> CGCATATTTGCG;> CGCAAAT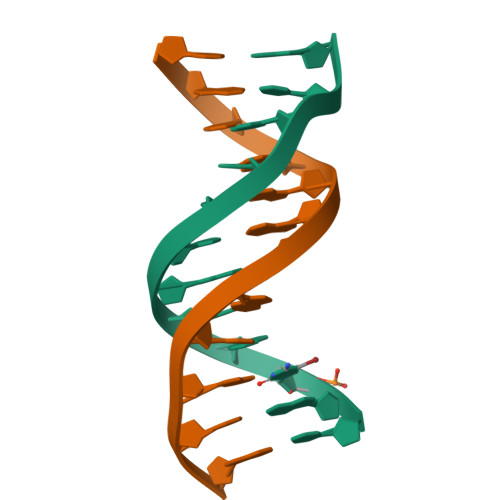ATGCG>FQGMATVSEVTYELLRARGLTTVFGNPGSNELPFLSGMPDDFRYVLGLHEGAVLSMADGYSLVTGEATLVNLHAASGSGNAMGALTNSVYSHSPLVVTAGQQVRSTIGQEVMLSNVDAGTLMKPLVKWSSEPTCAEDVPRTINQAIHTALLPAKGPVYVSVPYDDWAAEAPPESAGLLAREVHSAASLSGDQINDLIETLESATNPVLVLGPAVDADRANADAVLLAEKLRAPVWIAPSPSRCPFPTRHPSFRGVLPAGVADLSKTLEGHDLILVVGAPVFRYHQYVPGNYLPGGARLIHVTDDGGEAARAPIGEAYVAPVGSTLEILANMVKPSDRSPL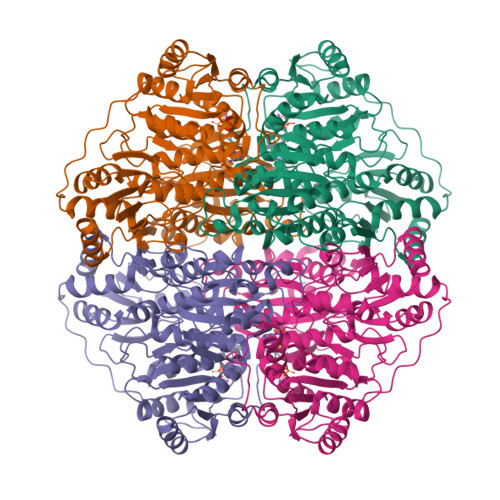PPLGDFEEAVSVGAGLDPAQLFALVRAGAPDDAIYVNESTSTSDAFWSQMDLSHQGSYYFPASGGLGFGLPAAVGAQLASPDRQVIGLIGDGSANYGITALWSAAQYKIPVVIIILNNGTYGALRGFSKILNTGETPGLDVPGIDFVHLAEGYGVRGTAVATAEDFTTAFKSALAADAPTLIEVRTNFDES[4x]>HMPAFLSKLWTLVEETHTNEFITWSQNGQSFLVLDEQRFAKEILPKYFKHNNMASFVRQLNMYGFRKVVHIDSGIVKQERDGPVEFQHPYFKQGQ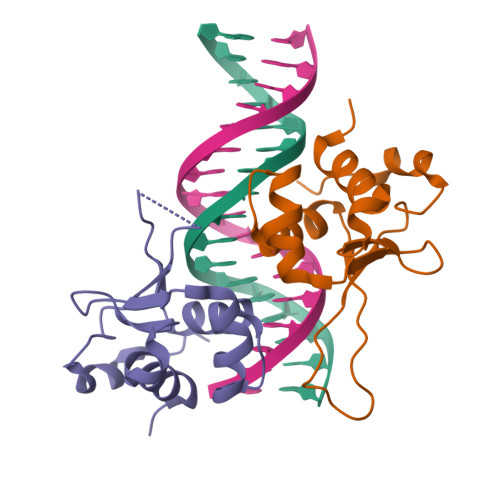DDLLENIKRKVSSSK[4x]> QDSLPDTKASGPAHSKEVPALTAVETGATNPLAPSDTVQTRHVVQRRSRSESTIESFFARGACVAIIEVDNEQPTTRAQKLFAMWRITYKDTVQLRRKLEFFTYSRFDMEFTFVVTANFTNANNGHALNQVYQIMYIPPGAPTPKSWDDYTWQTSSNPSIFYTYGAAPARISVPYVGLANAYSHFYDG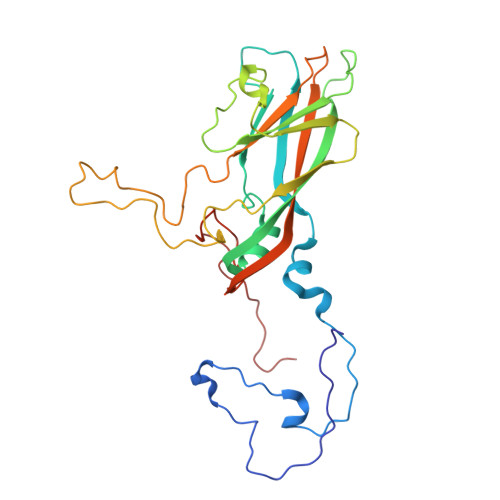FAKVPLKTDANDQIGDSLYSAMTVDDFGVLAVRVVNDHNPTKVTSKVRIYMKPKHVRVWCPRPPRAVPYYGPGVDYRNNLDPLSEKGLTTY> MFKNAKEFVQYANKLKTLREKKLNGVSIYVCVGTGCTAKGALKVYSAFEEELKKRNLLGQVTLEKIDDDKVTLNRTGCCGRCSSGPLVKIMPYRFFYSNVAPEDVPEIVDRTVLKGEPIERLFLTDPLTGEKVPRIEDTTLFKNQDFYIMEAIGESECDSIEDYIARSGYESLVKALTSMTPEEIIETVKASGLRGRGGGGFPTGLKWEFTRKAQGDIKFVVCNGDEGDPGAFMNRTLLERDPHLVLEGMIIAGYAVGAQKGYAYIRAEYPFAVKMFKKAIEDARKLGLLGENILGTGFSFDLEVKEGAGAFVCGEETALLASIEGKRGMPRPKPPFPAQSGLWGKPTLINNVETYANIPRILRDGVENYRKRGT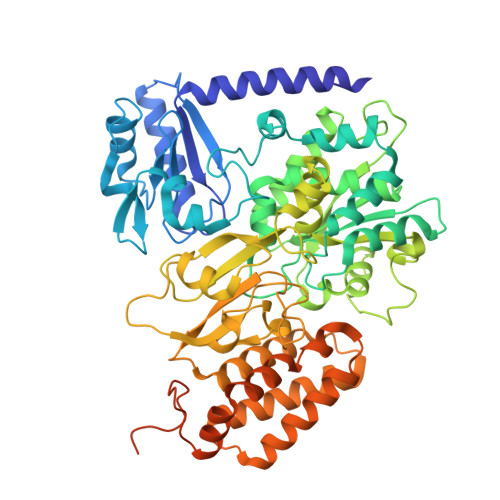ENSPGTKMFSVAGPLKATGIIEVEFGTTLRDIIYNICGGFVEGEEFKAVQIGGPSGACLSEDFIDMPLDYDTLKKADAMVGSGGIVVITKKTCMVEVARFFLDFTKRESCGKCVPCREGTMQAYNILEKFTHGKATYEDLKTLEHLSKTIKTASLCGLGKTAPNPILSTLKLFREEYIAHIEGECPSGMCTAFKKYVINPDICKGCGLCARSCPQNAITGERGKPYTIDQEKCVKCGLCASKCPFKAIELV>MLRFAVLGHPVAHSLSPAMHAFALESLGLEGSYEAWDTPLEALPGRLKEVRRAFRGV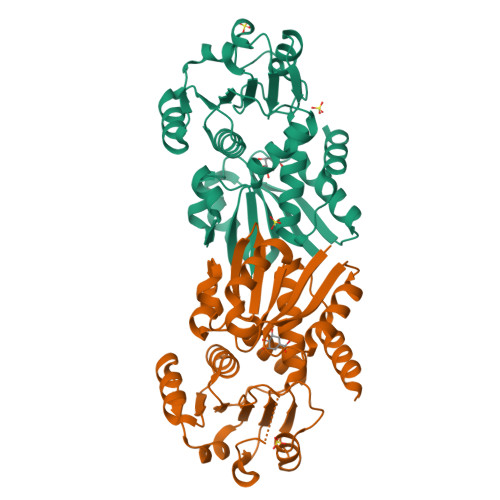NLTLPLKEAALAHLDWVSPEAQRIGAVNTVLQVEGRLFGFNTDAPGFLEALKAGGIPLKGPALVLGAGGAGRAVAFALREAGLEVWVWNRTPQRALALAEEFGLRAVPLEKAREARLLVNATRVGLEDPSASPLPAELFPEEGAAVDLVYRPLWTRFLREAKAKGLKVQTGLPMLAWQGALAFRLWTGLLPDPSGMEEAARRALGV[2x]>[4x]SNA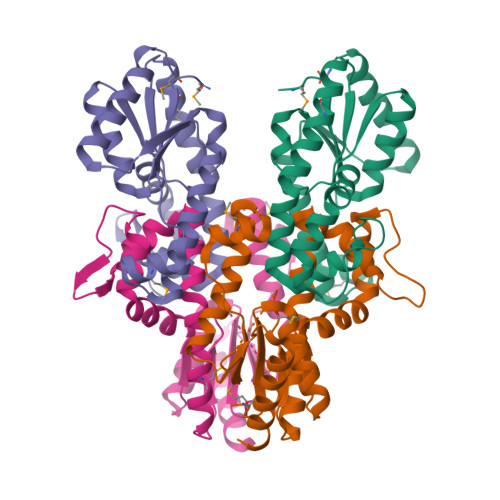MKNAFFVTASIACGKSTFIEIANSLGFKSISADKIAHKILDENALELEKIFSPFSLKNLLKKEKKIDRKILGEIVFNNKEAKKILENFTHPKIRAKILEQMQILDKENKAFFVEIPLFFESGAYENLGKVIVIYTPKELSLKRIMQRDKLSLEAAKARLDSQIDIEEKLKKADFIIKNTNSYADFRQECVKVIQEISKGNM> MNTGSFFINHEHDWQDVEPGIQRKIVAHTPDLMAVCVKFDRGAVGTPHQHERHDQIGYVVQGAFEVELEGEKRRLSPGDAFVAPHHTMHGAVALEPDSLVIDLFSP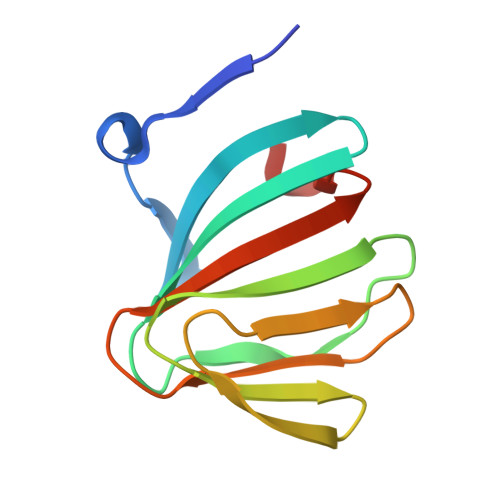RRDDMLKS> MARQNLKSTDRAVQQMLDKAKREGIQTVWDRYEAMKPQCGFGETGLCCRHCLQGPCRINPFGDEPKVGICGATAEVIVARGLDRSIAAGA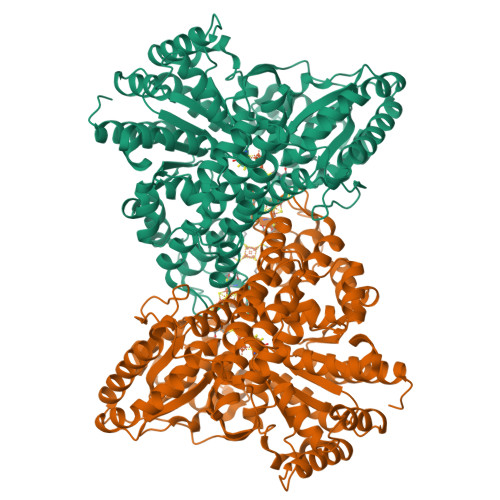AGHSGHAKHLAHTLKKAVQGKAASYMIKDRTKLHSIAKRLGIPTEGQKDEDIALEVAKAALADFHEKDTPVLWVTTVLPPSRVKVLSAHGLIPAGIDHEIAEIMHRTSMGCDADAQNLLLGGLRCSLADLAGCYMGTDLADILFGTPAPVVTESNLGVLKADAVNVAVHGHNPVLSDIIVSVSKEMENEARAAGATGINVVGICCTGNEVLMRHGIPACTHSVSQEMAMITGALDAMILDYQCIQPSVATIAECTGTTVITTMEMSKITGATHVNFAEEAAVENAKQILRLAIDTFKRRKGKPVEIPNIKTKVVAGFSTEAIINALSKLNANDPLKPLIDNVVNGNIRGVCLFAGCNNVKVPQDQNFTTIARKLLKQNVLVVATGCGAGALMRHGFMDPANVDELCGDGLKAVLTAIGEANGLGGPLPPVLHMGSCVDNSRAVALVAALANRLGVDLDRLPVVASAAEAMHEKAVALGTWAVTIGLPTHIGVLPPITGSLPVTQILTSSVKDITGGYFIVELDPETAADKLLAAINERRAGLGLPW>MASAEDVVVVNKQVLLKHFIPEGAPKETDMELVTTGTIRLRVPEGSNAVLLKNLYLSCDPYMRMRMTKHEEASYVDDFVPGAPITGFGVGKVVDSSHPDFKTGDYVWGLIGWEEYSLITKPQGLFKIHHTEIPLSYYTGILGMVGLTAYVGFYDICSPKKGERVFVSAAAGAVGQIVGQFAKQFGCYVVGSAGSDEKVNLLKTKFGFDEAFNYKKEPDLTKALKRYFPEGIDIYFENVGGPMLEAVLHNMRIKGRIAACGMISQYNLE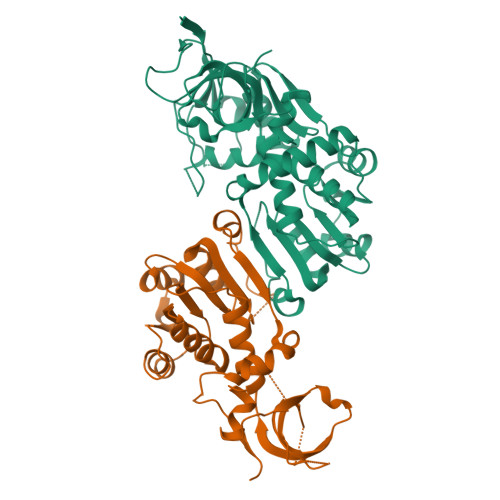KPEGVHNLFLIVGKRIRLEGFLVFDHYGSYPEFEEKVVQLIKEEKIKYLEDIVEGLENAPAALIGLFEGRNVGKQVVVVSREKGHHHHHH[4x]>MGAAAGERRTLSRKRGTTVDVPVKQESRQDRFEDQDEDRFAAQESIECSRLGDGIALAEFSGAHEQNPFSRARMRELTALMRELDADEKVRCVVLYGGAGRSFGVGGDFHEVSEFTGGDEVNAWIDDITDLYTTVAAISKPVIAAIDGYAIGVGLQISLCCDYRLGSEQARLVMPEFRVGIACNFGGFM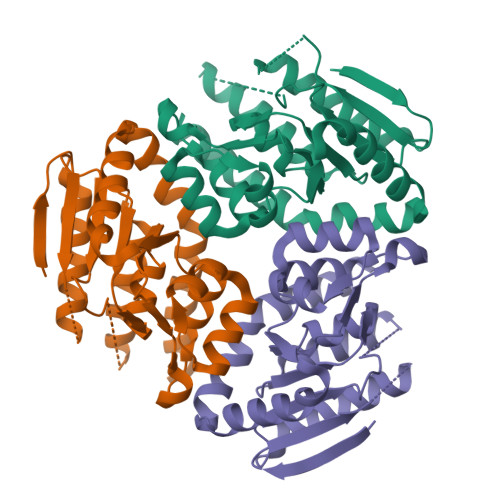LEAAAGRTVMQRMLLTCDEWPAERALADGLLHETVASPRLLDRALELARTISGYTAEAVQSTRPRVNAPFVAGLERIRREAKESHRRAFAAGEAQVRMRRVIGRS[3x]>[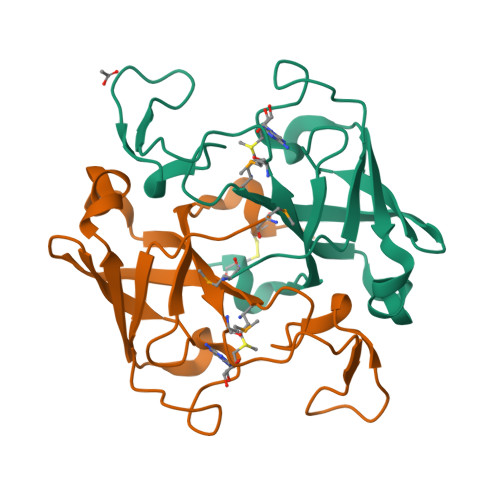2x]MILKPIGVVKSPFKTQNDAPRQGRFSDAVSEIAIFDEYADGLHKIENLRHIIVLYWMDKASRDKLRVVPPGETEERGVFTTRSPSRPNPIGLCVVEILEVERNRLKVRWLDALDGSPVIDIKKYSPEIDCVNQLEGQQPLEHHHHHH> MKTEWPELVGKSVEEAKKVILQDKPEA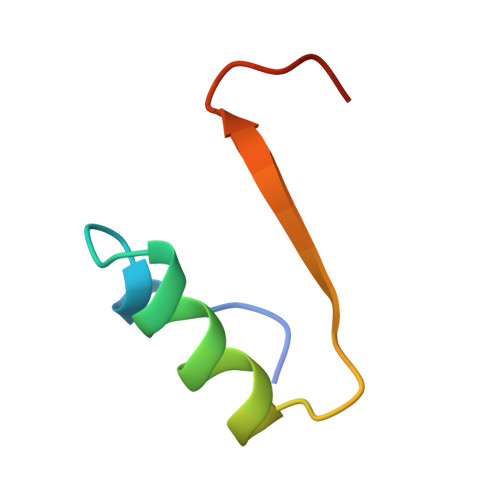QIIVLPVGTIVTM> GSMADEATRRVVSEIPVLKTNAGPRDRELWVQRLKEEYQSLIRYVENNKNADNDWFRLESNKEGTRWFGKCWYIHDLLKYEFDIEFDIPITYPTTAPEIAVPELDGKTAKMYRGGKICLTDHFKPLWARNVPKFGLAHLMALG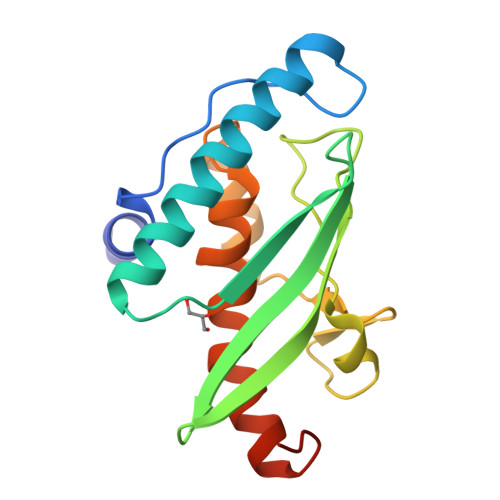LGPFLAVEIPDLIQKGVIHHKEKCNQ>MGSSHHHHHHSSGENLYFQGHMPEAVVIDGRAVAKAIQKELTEEVALLERRYKGRRPGLSTIICGKRKDSQTYVRLKRKAAAACGFRNFSVELPANVTQEALEREVIRLNEEEAC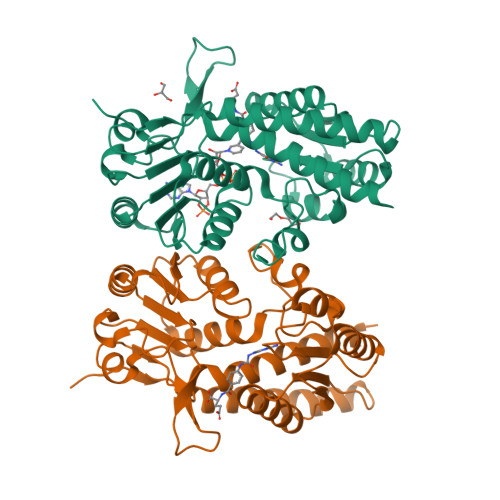HSIVVQLPLPPHIDKVAALSKIKPEKDADCLLPVNVGQLHIRERNPAIVPCTASAVMELLRCSGVEICGKRVVVLGRGDIAGLPVATLLANEDATVTVVHSATPLCDIADIVRASDIVVSAAGQPGLVRGEWIKLGAAVIDVGTTPVADPSKVPGYRLVGDVCFDVARKRAAYITPVPGGVGPVTVSMLLKNTLTMFKRSVRAL[2x]> GSSPEKPTPNGGIPHDNLVLIRMKPDENGRFGFNVKGGYDQKMPVIVSRVAPGTPADLCVPRLNEGDQVVLINGRDIAEHTHDQVVLFIKASCERHS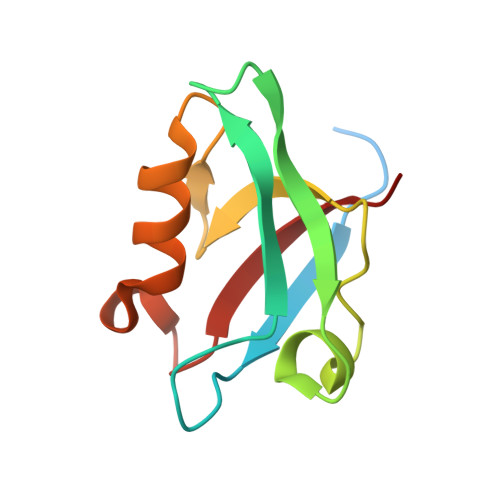GELMLLVRPN>MKELI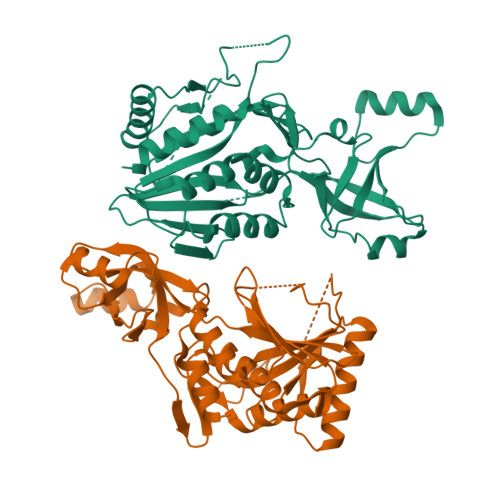RKLTEAFGPSGREEEVRSIILEELEGHIDGHRIDGLGNLIVWKGSGEKKVILDAHIDEIGVVVTNVDDKGFLTIEPVGGVSPYMLLGKRIRFENGTIGVVGMEGETTEERQENVRKLSFDKLFIDIGANSREEAQKMCPIGSFGVYDSGFVEVSGKYVSKAMDDRIGCAVIVEVFKRIKPAVTLYGVFSVQEEVGLVGASVAGYGVPADEAIAIDVTDSADTPKAIKRHAMRLSGGPALKVKDRASISSKRILENLIEIAEKFDIKYQMEVLTFGGTNAMGYQRTREGIPSATVSIPTRYVASPSEMIAPDDVEATVDLLIRYLGA[2x]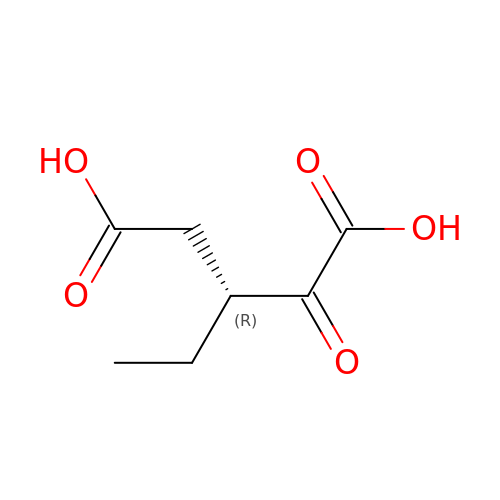(3~{R})-3-ethyl-2-oxidanylidene-pentanedioic acid | C7 H10 O5 | SWPMNQDYIMXOTM-SCSAIBSYSA-N>SMTFGQALESLKRGHLVARKGWNGKGMFIFMRPEDSLPTNMIVNQVKSLPESFKRWVANNHGDSETDRIKFTAYLCMKAADGTIVNGWLASQTDMLANDWVI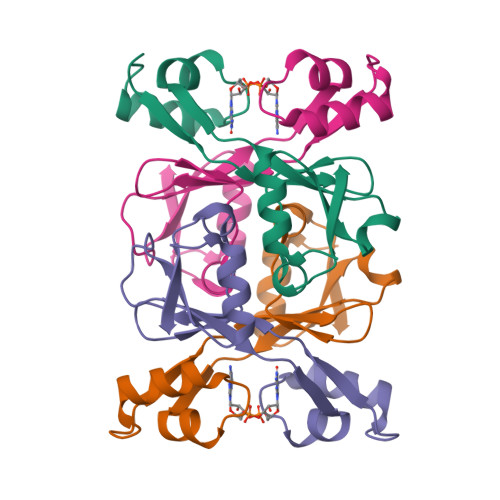VE[4x]> MQNSALKAWLDSSYLSGANQSWIEQLYEDFLTDPDSVDANWRSTFQQLPGTGVKPDQFHSQTREYFRRLAKDASRYSSTISDPDTNVKQVKVLQLINAYRFRGHQHANLDPLGLWQQDKVADLDPSFHDLTEADFQETFNVGSFASGKETMKLGELLEALKQTYCGPIGAEYMHITSTEEKRWIQQRIESGRATFNSEEKKRFLSELTAAEGLERYLGAKFPGAKRFSLEGGDALIPMLKEMIRHAGNSGTREVVLGMAHRGRLNVLVNVLGKKPQDLFDEFAGKHKEHLGTGDVKYHMGFSSDFQTDGGLVHLALAFNPSHLEIVSPVVIGSVRARLDRLDEPSSNKVLPITIHGDAAVTGQGVVQETLNMSKARGYEVGGTVRIVINNQVGFTTSNPLDARSTPYCTDIGKMVQAPIFHVNADDPEAVAFVTRLALDFRNTFKRDVFIDLVCYRRHGHNEADEPSATQPLMYQKIKKHPTPRKIYADKLEQEKVATLEDATEMVNLYRDALDAGDCVVAEWRPMNMHSFTWSPYLNHEWDEEYPNKVEMKRLQELAKRISTVPEAVEMQSRVAKIYGDRQAMAAGEKLFDWGGAENLAYATLVDEGIPVRLSGEDSGRGTFFHRHAVIHNQSNGSTYTPLQHIHNGQGAFRVWDSVLSEEAVLAFEYGYATAEPRTLTIWEAQFGDFANGAQVVIDQFISSGEQKWGRMCGLVMLLPHGYEGQGPEHSSARLERYLQLCAEQNMQVCVPSTPAQVYHMLRRQALRGMRRPLVVMSPKSLLRHPLAVSSLEELANGTFLPAIGEIDELDPKGVKRVVMCSGKVYYDLLEQRRKNNQHDVAIVRIEQLYPFPHKAMQEVLQQFAHVKDFVWCQEEPLNQGAWYCSQHHFREVIPFGASLRYAGRPASASPAVGHMSVHQKQQQDLVNDALNVE;> MQNSALKAWLDSSYLSGANQSWIEQLYEDFLTDPDSVDANWRSTFQQLPGTGVKPDQFHSQTREYFRRLAKDASRYSSTISDPDTNVKQVKVLQLINAYRFRGHQHANLDPLGLWQQDKVADLDPSFHDLTEADFQETFNVGSFASGKETMKLGELLEALKQTYCGPIGAEYMHITSTEEKRWIQQRIESGRATFNSEEKKRFLSELTAAEGLERYLGAKFPGAKRFSLEGGDALIPMLKEMIRHAGNSGTREVVLGMAHRGRLNVLVNVLGKKPQDLFDEFAGKHKEHLGTGDVKYHMGFSSDFQTDGGLVHLALAFNPSHLEIVSPVVIGSVRARLDRLDEPSSN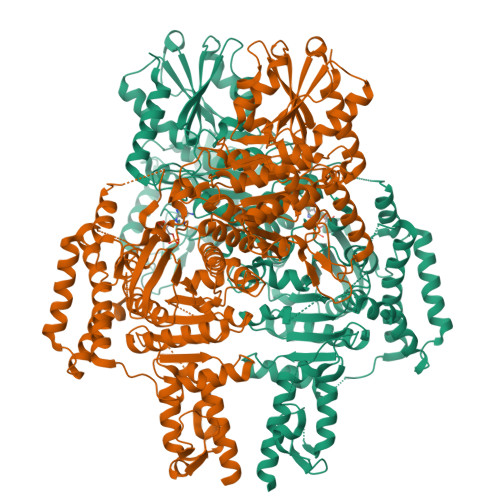KVLPITIHGDAAVTGQGVVQETLNMSKARGYEVGGTVRIVINNQVGFTTSNPLDARSTPYCTDIGKMVQAPIFHVNADDPEAVAFVTRLALDFRNTFKRDVFIDLVCYRRHGHNEADEPSATQPLMYQKIKKHPTPRKIYADKLEQEKVATLEDATEMVNLYRDALDAGDCVVAEWRPMNMHSFTWSPYLNHEWDEEYPNKVEMKRLQELAKRISTVPEAVEMQSRVAKIYADRQAMAAGEKLFDWGGAENLAYATLVDEGIPVRLSGEDSGRGTFFHRHAVIHNQSNGSTYTPLQHIHNGQGAFRVWDSVLSEEAVLAFEYGYATAEPRTLTIWEAQFGDFANGAQVVIDQFISSGEQKWGRMCGLVMLLPHGYEGQGPEHSSARLERYLQLCAEQNMQVCVPSTPAQVYHMLRRQALRGMRRPLVVMSPKSLLRHPLAVSSLEELANGTFLPAIGEIDELDPKGVKRVVMCSGKVYYDLLEQRRKNNQHDVAIVRIEQLYPFPHKAMQEVLQQFAHVKDFVWCQEEPLNQGAWYCSQHHFREVIPFGASLRYAGRPASASPAVGYMSVHQKQQQDLVNDALNVE>MHIIPVASDPKTCSSGVNENSLDFDFTMAFQPIVNCRTKEIFGYEALVRGLNNESAYSVISRVNEDNRYLFDQMCRVKAIALAAKLGLTSKLSINFLPNAIYVPERCIRTTLEAAKRYQFPIENIMFEFTEAERVEDVN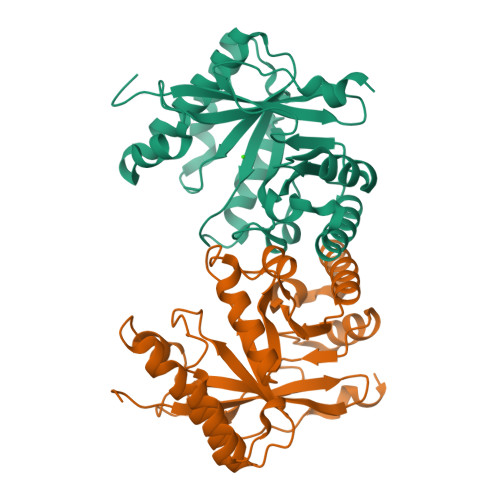HIKRIVEYYKSLGFQTAIDDFGSGYSGLNLLADFQTNIVKVDMGLIRNIHADQVRQSIMKNCLKLFSDLNIQPLAEGVESHAEFAWLKAAGVELMQGYYFAKPGFESLPSVNPEFSEA[2x]> ETGTPMMPPVGVQASILSHDTIRITWADNSLPKHQKITDSRYYTVRWKTNIPANTKYKNANATTLSYLVTGLKPNTLYEFSVMVTKGRRSSTWSMTAHGATFELVPTSPPKDVTVVSKEGKPRTIIVNWQPPSEANGKITGYIIYYSTDVNAEIHDWVIEPVVGNRLTHQIQELTLDTPYYFKIQARNSKGMGPMSEAVQFR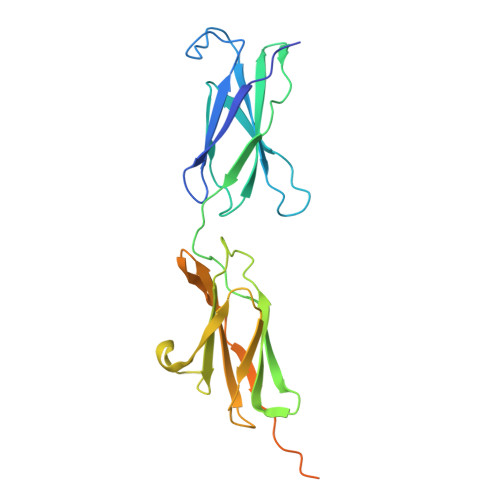TPKALGSAGKGSRLPDLGSDYKPPMSGSNSPHGSPTSPLDSNGTKHHHHHH> CAAAGAAAAG;> CTX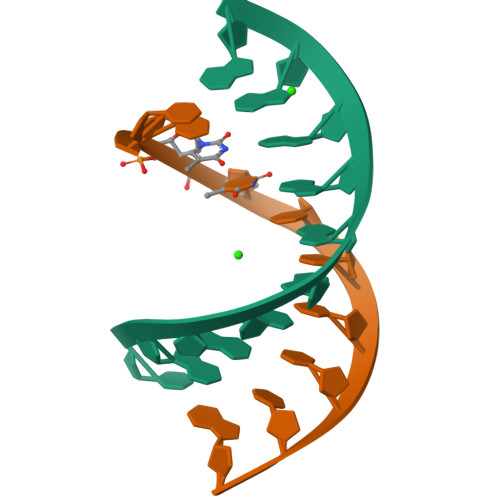TCTTTG> GSPGISGGGGGSHIEGYECQPIFLNVLEAIEPGVVCAGHDNNQPDSFAA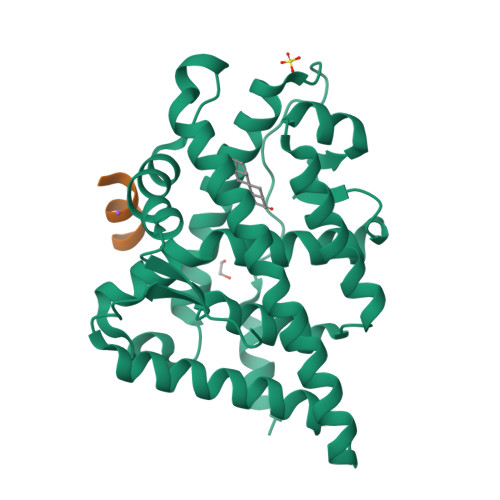LLSSLNELGERQLVHVVKWAKALPGFRNLHVDDQMAVIQYSWMGLMVFAMGWRSFTNVNSRMLYFAPDLVFNEYRMHKSRMYSQCVRMRHLSQEFGWLQITPQEFLCMKALLLFSIIPVDGLKNQKFFDELRMNYIKELDRIIACKRKNPTSCSRRFYQLTKLLDSVQPIARELHQFTFDLLIKSHMVSVDFPEMMAEIISVQVPKILSGKVKPIYFHTQ;> SRWAEVWDDNSKVSR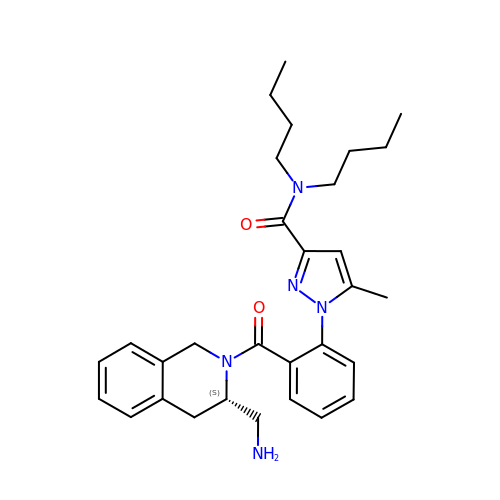1-[2-[[(3~{S})-3-(aminomethyl)-3,4-dihydro-1~{H}-isoquinolin-2-yl]carbonyl]phenyl]-~{N},~{N}-dibutyl-5-methyl-pyrazole-3-carboxamide | C30 H39 N5 O2 | CLINUOVVDXSAST-VWLOTQADSA-N2-acetylamino-2-deoxy-alpha-L-idopyranose | C8 H15 N O6 | 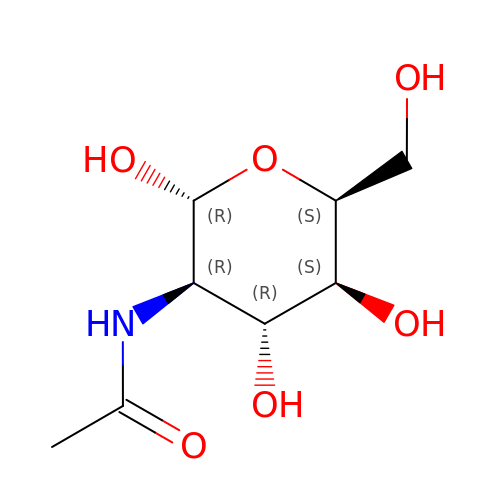OVRNDRQMDRJTHS-SLBCVNJHSA-N> MESRGGGGRVRLPGTTMQDNIRFVSAGDDVKIWDYSSMTTVEQFNPHSASHPVSSLCWSSNNHFLVTASGSGDKIVVSSCKSKPVPLLELAEGKKQTCVNLNSSSQYVVSGGLDNTVNIWDLKSKRLHRSLKDHKDEVTCVTFNANDCYVASGSMSGEIILHNVTTNLSSTPFGHGSSQPIRHLKYSYVKKSLLGTVSDSGSVTLWDANSQNPYHVFESAHKAPASGICFSPVNDLLLVTVGLDKRIICYDVSSKILLQTVVAESPLTAVDFMPDGATLAVGSSRGKIYLYDLRMLSSPVKTVSAHKTSVQCIQFQHSNIYKSSKGPSSKSSILSTAVNKKPSTKTAAGGTQSANITKDLPPSAISSLPQPVMPVDSKVLRVNDDKSGFPRSTSLDIIPSKETDFAKTSDYKSIDSFGRSSLGDIFSPVRDDASHFRGAEDLSCKGNDLDYLPQFSTIPSSRRNPVGANTQGIHGSPLHLIIESPIKEEDESQDSELKTRKPQLLKQDFRESSSKPASVDQNNLNNSPINSVTRTPEAIEKTGHQILSQLKSDVPAHGTKIASPKVAATMSTQLASSLSEKIADTLASDRTGAPLTAIQINFIKNMIEETLDDFREACHRDIVNLQVEMI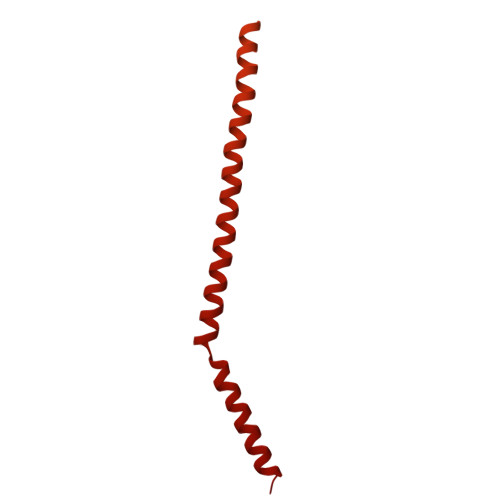KQFHIQSSEIQMLLERYSLNESLVSEIEKLREENKRLRANF> HHHHHHSQDPMNALTTIDFNQHVIVRLPSKNYKIVELKPNTSVSLGKFGAFEVNDIIGYPFGLTFEIYYDGEEVSSDENRDSKPKNKIPIGKVRLLSQEIKDVNNDKDDGQSEPPLSIKEKSVSLELSSIDSSATNQNLVNMGSKAQELTVEEIEKMKQESLSSKEIIDKIIKSHKSFHNKTVYSQEKYVNRKKQKFAKYFTVEYLSSSNLLQFLIDKGDIQRVLDMSQESMGMLLNLANIQSEGNYLCMDETGGLLVYFLLERMFGGDNESKSKGKVIVIHENEHANLDLLKFANYSEKFIKEHVHTISLLDFFEPPTLQEIQSRFTPLPKEEARALKGGKKNSYYRKLRWYN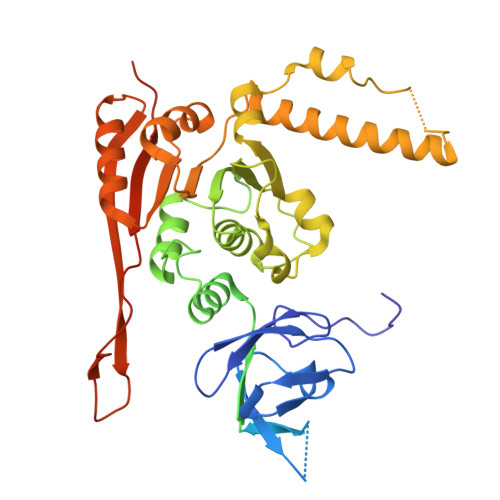TQWQILELTGEFLYDGLVMATTLHLPTLVPKLAEKIHGSRPIVCYGQFKETLLELAHTLYSDLRFLAPSILETRCRPYQSIRGKLHPLMTMKGGGGYLMWCHRVIPAPEPVSENATAADSSEKLAEHGAKKQKI>[2x]DYKDDDDKLAAAQYPVVNTNYGKIRGLRTPLPNEILGPVEQYLGVPYASPPTGERRFQPPEPPSSWTGIRNTTQFAAVCPQHLDERSLLHDMLPIWFTANLDTLMTYVQDQNEDCLYLNIYVPTEDDIHDQNSKKPVMVYIHGGSYMEGTGNMIDGSILASYGNVIVITINYRLGILGFLSTGDQAAKGNYGLLDQIQALRWIEENVGAFGGDPKRVTIFGSGAGASCVSLLTLSHYSEGLFQKAIIQSGTALSSWAVNYQPAKYTRILADKVGCNMLDTTDMVECLRNKNYKELIQQTITPATYHIAFGPVIDGDVIPDDPQILMEQGEFLNYDIMLGVNQGEGLKFVDGIVDNEDGVTPNDFDFSVSNFVDNLYGYPEGKDTLRETIKFMYTDWADKENPETRRKTLVALFTDHQWVAPAVATADLHAQYGSPTYFYAFYHHCQSEMKPSWADSAHGDEVPYVFGIPMIG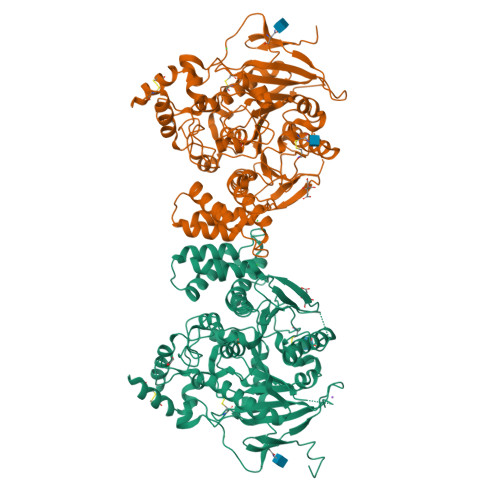PTELFSCNFSKNDVMLSAVVMTYWTNFAKTGDPNQPVPQDTKFIHTKPNRFEEVAWSRYNPKDQLYLHIGLKPRVRDHYRATKVAFWLELVPHLHNLNEIFQYVSTTTKVPPPDMT> LAHSKMVPIPAGVFTMGTDDPQIKQDGEAPARRVTIDAFYMDAYEVSNTEFEKFVNSTGYLTEAEKFGDSFVFEGMLSEQVKTNIQQAVAAAPWWLPVKGANWRHPEGPDSTILHRPDHPVLHVSWNDAVAYCTWAGKR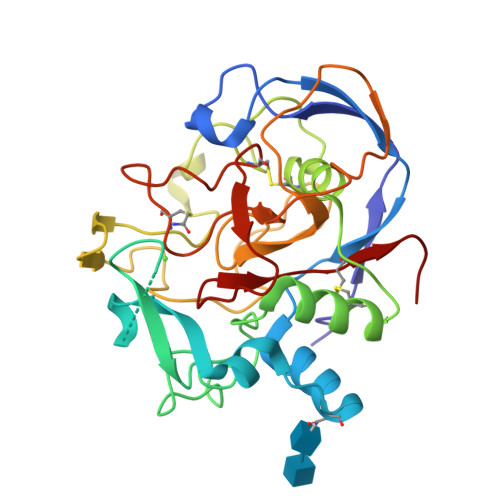LPTEAEWEYSCRGGLHNRLFPWGNKLQPKGQHYANIWQGEFPVTNTGEDGFQGTAPVDAFPPNGYGLYNIVGNAWEWTSDWWTVHHSVEETLNPKGPPSGKDRVKKGGSYMCHRSYCYRYRCAARSQNTPDSSASNLGFRCAADRLP> MEQFKQFSIEKQAAINSLLQLRGMLEMLGEMGINISDDLQKVTSAINAIESDVLRIALLGAFSDGKTSVIAAWLGKVMDDMNISMDESSDRLSIYKPEGLPDQCEIVDTPGLFGDKEREVDGRLVMYEDLTRRYISEAHLIFYVVDATNPLKESHSDIVKW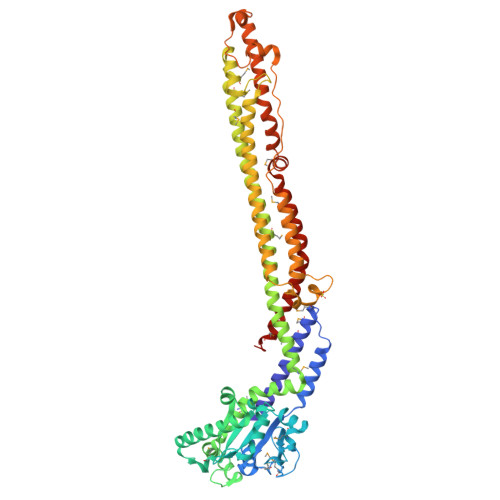VLRDLNKLSSTIFVINKMDEVTSLTDQALFDEQAAIKKANLKGKLQRAADLTAQECEQLNIVCVASNPNGRGLTYWFTKPEHYESRSRINDLKNAATEILKTNVPEVLLVKTGMDVVKDIVIQRVTLASRHLDELNTFVEKNDEDMHRFSNDIKQSRIEVKRLAGELFEELNLMEKQLMSQLRPLDLDDIRPFMDDELGYTEDGVGFKLHLRIKQSVDRFFEQSTAVSQRLSDDITRQLSSSESFLSGLGEGAFRSLGGAFKGVSKISPATLKTTILAARDTIGKLTGYVYKFKPWEATKLAGSIAKWAGPVGAAFTIGSDLWDAYKAHEREQELKEVKASLAKIIKEPFEDIYDVLSSDEKMFAFFAPQIQQMEQVVTELAEKSQAIRDNRQKLSLIQTQLAQLMVPATENHTAR>[2x]GPMRRSYEGYKVYGIVPESPDEAEILYQIRQSNPDLDFWHLTKQPGDEARVLVAPKDQRSFLIKLIRHGLHYQEVISDVEGTLAPYNEPRTRGMSLDR;>[2x]DVSTSYLRHNEINEYLQTLSQKYPSLVSVEEAGTSYEGRSIKTITINKKPGNAVVFLDAGIHAREWIAPATALYAIEQLVEHSSENQEVLSNLTWVIMPVVNPDGYEFSHETDRFWRKTRKPTGKSCKGTDGNRNFDYHWGEVGASTQACADTFRGETAFSEPETRAVRDAVMKLKGSCKFYLSLHSYGNYILYPWGWTSKLPETWEAIDEVAQAGAEAIKQSTGSRYTVGSSTNVLYAAAGGSDDWAFAVAEVPISITMELPGGGNGGFNPPPSSIEKIVNESWVGIKAMALKVAQMF

In mosquitoes, the A/B subfamily of MCPs (including carboxypeptidases A and B; CPB and CPA, respectively) is primarily responsible for dietary blood digestion for the release of amino acid–rich nutrients required for egg development. In the midgut of Ae. aegypti mosquito, procarboxypeptidase B1 (CPB1 or PCPBAe1) takes on a different role in pathogen infection, interacting with the DENV-2 envelope (E) protein/virion and impeding viral packaging, maturation, and release from the midgut. Based on sequence analyses, PCPBAe1 is expressed as a preproprotein, with a signal peptide (Met*–Ala*), an N-terminal pro-region (Ala1A–Asp75A; “A” to indicate the activation unit or pro-region), and a C-terminal mature peptidase domain (Asp7–Phe305) (CPBAe1). Here, we report the crystal structure of Aedes aegypti procarboxypeptidase B1 (PCPBAe1), characterized its substrate specificity and mechanism of binding to and inhibiting Dengue virus (DENV).

Here, we characterized the enzymatic activity of the mature peptidase domain (CPBAe1) and determined the structure of the full-length (FL)-PCPBAe1 (proenzyme) at 2.08-Å resolution. However, the structure consists of two molecules in the asymmetric unit of the crystal. The activation loop (Asp75A–Asp7) that connects the pro-region to the mature peptidase domain is disordered and could not be modeled in our structure. The pro-region adopts an open-sandwich antiparallel-α/antiparallel-β-fold, consisting of two α-helices and four β-strands. The mature peptidase domain contains a zinc-coordinated active site triad and the substrate-binding pocket and displays a core of eight twisted β-sheets surrounded by eight α-helices. One zinc atom is present in each molecule of the structure and forms pentahedral coordination with the catalytic residues: His68Nδ1, His192Nδ1, Glu71Oε1, and Oε1 atoms and a water molecule. CPBAe1 contains one disulfide bond (Cys133–Cys156), which is the only conserved disulfide bond present in MCPs. Moreover, CPBAe1 displays two of the three cis-peptide bonds (Ser193–Tyr194 and Pro201–Trp202) present in mammalian MCPs. The globular N-terminal pro-region occupies the wide active site cleft of the mature peptidase domain, mediated via interactions with residues from the substrate-binding pocket of the peptidase region. Residues Asp34A and Phe35A from the pro-region make contacts with the S2 subsite residue Arg70; this interaction is crucial for blocking small-peptide substrates from contacting the zinc atom, and thus maintain PCPBAe1 in its inactive form.> CLGTIGPVTPLDASDFALDIRMPGVTPKESDTYFCMSMRLPVDEEAFVIDFKPRASMDTVHHMLLFGCNMPSSTGSYWFCDEGTCTDKANILYAWARNAPPTRLPKGVGFRVGGETGSKYFVLQVHYGDISAFRDNHKDCSGVSVHLTRVPQPLIAGMYLMMSVDTVIPPGEKVVNADISCQYKMY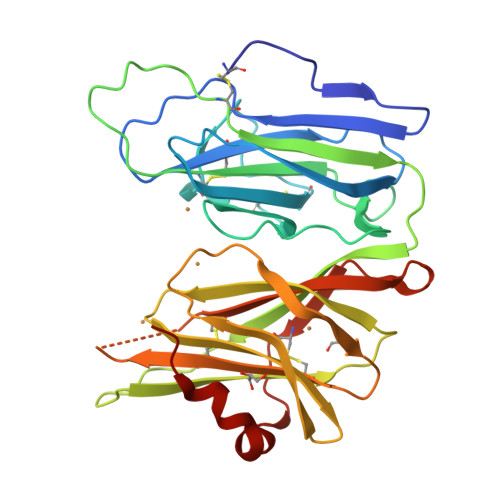PMHVFAYRVHTHHLGKVVSGYRVRNGQWTLIGRQNPQLPQAFYPVEHPVDVTFGDILAARCVFTGEGRTEATHIGGTSSDEICNLYIMYYMEAKYALSFMTCTKNVAPDMFRTIPAEANIPIP> STENEKSRSLPAERNPLYKDDTLDHTPLIPKCRAQVIEFPDGPATFVRLKCTNPESKVPHFLMRMAKDSSISATSMFRSAFPKATQEEEDLEMRWIRDNLNPIEDKRVAGLWVPPADALALAKDYSMTPFINALLEASST;> GPLSDNEEFENVVKNGH

Bqt4 is one of the most abundant INM proteins in fission yeast Schizosaccharomyces pombe, and plays crucial roles in chromosome-NE association by interacting with different protein partners. Here, we report the crystal structures of the N-terminal domain of Bqt4 in complexes with Bqt4-binding motifs from Rap1, Lem2, and Sad1. The Bqt4NTD comprises six α helices and six β strands arranged in a compact α/β fold. Overall, our data suggest that Bqt4NTD is a protein-interaction module that recognizes a consensus motif.

Notably, Rap1BBM and Lem2BBM share a common sequence feature: three to four consecutive acidic residues followed by x-F-x-x-x-Φ (Φ stands for hydrophobic residues). Among these proteins, Sad1 has been shown to interact with Bqt1, and mediates the attachment of telomeres to the NE during meiosis. A 14-residue fragment of Sad1 (residues 88–101), referred to as Sad1BBM, can bind Bqt4NTD with the dissociate constant of 3.7 μM, as shown by ITC assays. We further determined the crystal structure of Bqt4NTD-Sad1BBM complex, and found that Bqt4NTD–Sad1BBM structure is virtually same as Bqt4NTD–Rap1BBM and Bqt4NTD–Lem2BBM structures. Sad1BBM interacts with Bqt4NTD in the same manner as that in Bqt4NTD–Rap1BBM and Bqt4NTD–Lem2BBM complexes. Mutations of the critical Bqt4 residues, including F46, F61, and R48, did not affect Sad1 stability, but severely impeded the interaction with Sad1BBM. Sad1 is localized to spindle pole body (SPB) and plays important roles in meiotic telomere bouquet formation. For example, S88 of Sad1, at the N-terminus of Sad1BBM, had been reported to be phosphorylated in three phosphoproteomics analyses.>MAGNADYNLTGFSQGNTGGGVISESNTAVYKKVYNATDLALALKKNSGVKVVEIMNDLNLGWNEIPSAAQTSPFAKHNDALTHPVLKQTGVSKITVDGFNGLTIFSANGSKIKHAAISVKRSSNVIIRNLEFDELWEWDESTKGDYDKNDWDYITLEESSGVWIDHCVFNKAYDGLVDSKKGTSGVTISWSTFKGDDGSPNSWVTRQINEMEANKASYPMYNYLRSSAVGLSKEDIIAISGSQKKGHLVGATSDESANANLSITLHHNVYKDIQDRMPRLRGGNAHAYNIIMDATDARAAQTRITS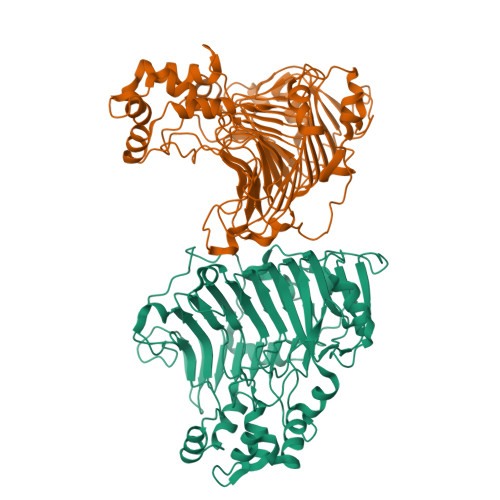GMAAAIASKGYKFGITSNGAISTESNAVLVEKSVIKDVQYPVRNNQTDPTNATYTGKIRVADTIYSLDGSSFRGSRDTAGSPLAPVPAAIKPFSWNGFSILPYSYQLDDPSTLNARLTASNGAGAGKLSWSKDNWLKTSY[2x]>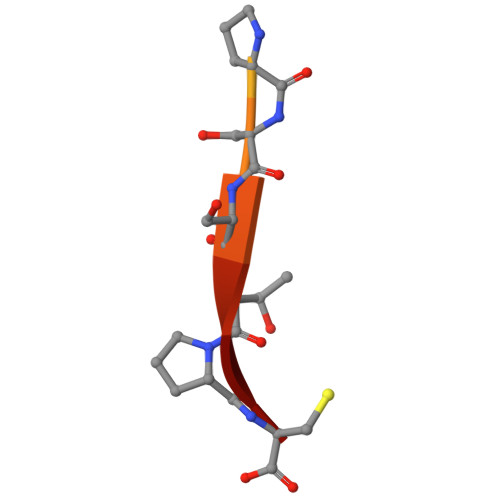 PPPPPPPPSSTPC>[2x]DLQIGFYNQSCPSAESLVQQGVAAAFANNSGIAPGLIRMHFHDCFVRGCDGSVLLDSTDTNTAEKDAAPNNPSLRGFEVIAAAKSAVEAACPKTVSCADILAFAARDSAALAGNITYQVPSGRRDGNVSLASEALTNIPAPTFNATQLINSFAGKNLTADEMVTLSGAHSIGVSHCFSFLNRIYNFSNTSQVDPTLSSSYADLLRTKCPSNSTRFTPITVSLDIITPTVLDNRYYTGVQLTLGLLTSD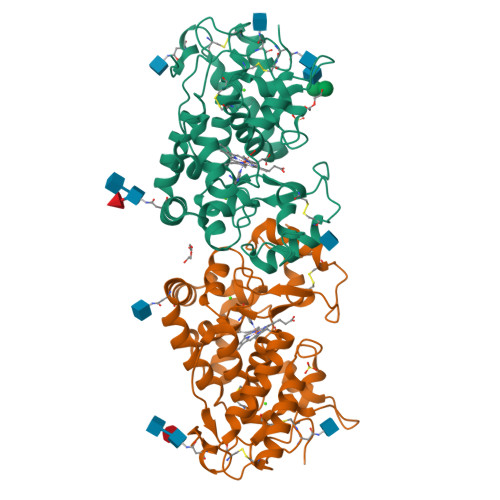QALVTEANLSAAVKNNADNLTAWVAEFAQAIVKMGQIEVLTGTQGEIRTNCSVVN tert-butyl 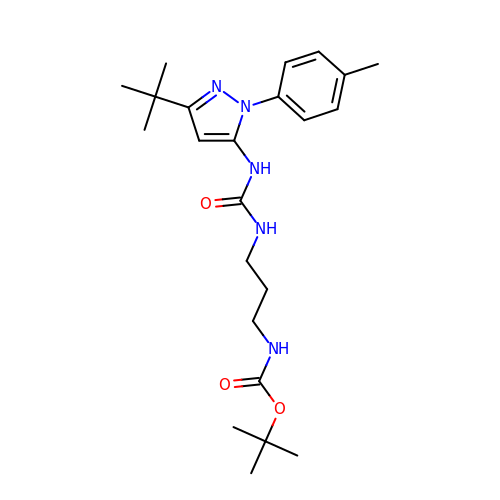[3-({[3-tert-butyl-1-(4-methylphenyl)-1H-pyrazol-5-yl]carbamoyl}amino)propyl]carbamate | C23 H35 N5 O3 | NTCPUSCJDOSUEX-UHFFFAOYSA-N>MGEKQQILDYIETNKYSYIEISHR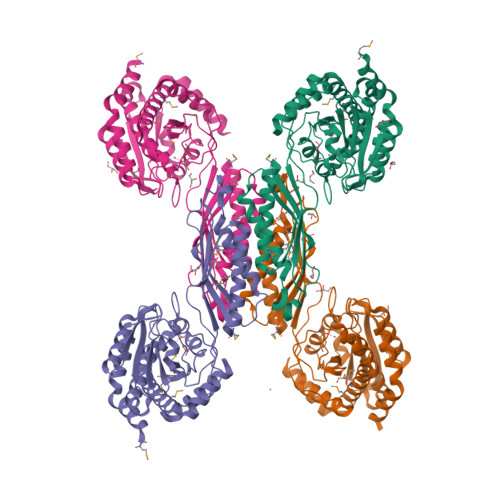IHERPELGNEEIFASRTLIDRLKEHDFEIETEIAGHATGFIATYDSGLDGPAIGFLAEYDALPGLGHACGHNIIGTASVLGAIGLKQVIDQIGGKVVVLGCPAEEGGENGSAKASYVKAGVIDQIDIALMIHPGNETYKTIDTLAVDVLDVKFYGKSAHASENADEALNALDAMISYFNGVAQLRQHIKKDQRVHGVILDGGKAANIIPDYTHARFYTRAMTRKELDILTEKVNQIARGAAIQTGCDYEFGPIQNGVNEFIKTPKLDDLFAKYAEEVGEAVIDDDFGYGSTDTGNVSHVVPTIHPHIKIGSRNLVGHTHRFREAAASVHGDEALIKGAKIMALMGLELITNQDVYQDIIEEHAHLKGNGK[4x]>ARMFEMFNLDWKSGGTMKIKGHISEDAESFAINLGCKSSDLALHFNPRFNESVIVCNSLCSDNWQQEQRDKHFNFYKGSTVKIIVEFLGDKFL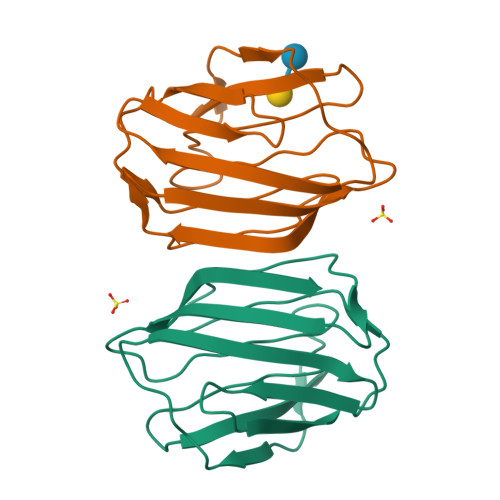VKLPDGHEVEFPNRHGYDKISYLNILGGFKVTSFKVE[6x]> SAMMYIQELRSGLRDMHLLSCLESLRVSLNNNPVSWVQTFGAEGLASLLDILKRLHDEKEETSGNYDSRNQHEIIRCLKAFMNNKFGIKTMLETEEGILLLVRAMDPAVPNMMIDAAKLLSALCILPQPEDMNERVLEAMTERAEMDEVERFQPLLDGLKSGTSIALKVGCLQLINALITPAEELDFRVHIRSELMRLGLHQVLQELREIE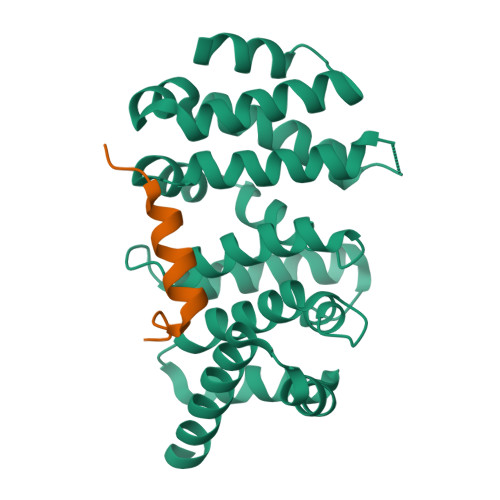NEDMKVQLCVFDEQGDEDFFDL;> DETGVMDSLLEALQSGAAFR> GSVDPLSVQGTGWMSKGQITVLDMHPGSGKTHRVLPELVRQCADRGMRTLVLAPTRVVLKEMERALAGKKVRFHSPAVEGQTTAGAIVDVMCHATYVHRRLLPQGRQNWEVAIMDEAHWTDPHSIAARGHLYSLAKENRCALVLMTATPPGRGDPFPESNGAIMSEERAIPDGEWREGFDWITEYEGRTAWFVPSISKGGAVARTLRQRGKSVICLNSKTFEKDYLRVREEKPDFVVTTDISEMGANLDVSRVIDGRT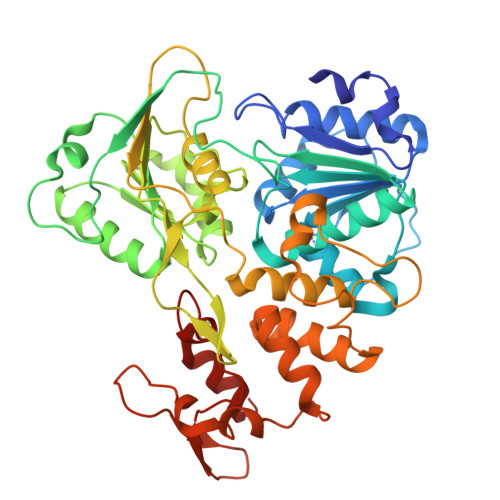NIKPEEVDGKVELTGTRKVTTASAAQRRGRVGRTSGRTDEYIYSGQCDDDDTSLVQWKEAQILLDNITTLRGPVATFYGPEQVKMPEVAGHYRLNEEKRKHFRHLMTQCDFTPWLAWHVATNTSNVLDRSWTWQGPEENAIDGADGDLVRFKTPGGSERVLQPVWKDCRMFREGRDVKDFILYASGRR> MNAHLANEVQYDLGHARVGPSSLVHVIISSECLAAAGIPLAALMRGRPGLGTAANFQVEIQTRAHATGDCTPWCTAFAAYVPADAVGELLAPVVPAHPGLLPRASSAGGLFVSLPVVCDAQGVYDPYAVAALRLAWGSGASCARVILFSYDELVPPNTRYAADSTRIMRVCRHLCRYVALLGAAAPPAAKEAAAHLSMGLGESASPRPQPLARPHAGAPADPPIVGASDPPISPEEQLTAPGGDTTAAQDVSIAQENEEILALVQRAVQDVTRRHPVRARTGRAACGVASGLRQGALVHQAVSGGAMGAADADAVLAGLEPPGGGRFVAPAPHGPGGEDILNDVLTLTPGTAKPRSLVEWLDRGWEALAGGDRPDWLWSRRSISVVLRHHYGTKQRFVVVSYENSVAWGGRRARPPLLSSALATALTEACAAERVVRPHQLSPAGQAELLLRFPALEVPLRHPRPVLPPFDIAAEVAFTARIHLACLRALGQAIRAALQGGPRISQRLRYDFGPDQRAWLGEVTRRFPILLENLMRAVEGTAPDAFFHTAYALAVLAHLGGRGGRGRRVVPLGDDLPARFADSDGHYVFDYYSTSGDTLRLNNRPIAVAMDGDVSKREQSKCRFMEAVPSTAPRRVCEQYLP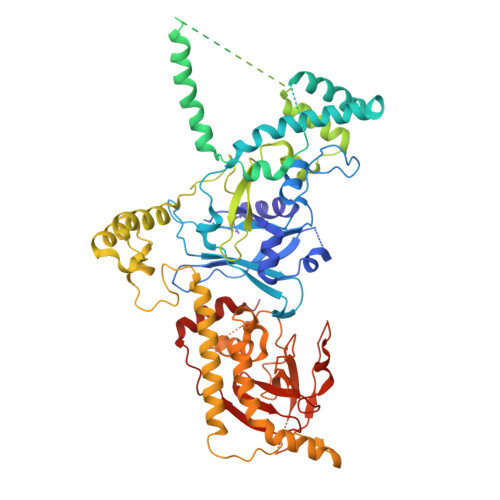GESYAYLCLGFNRRLCGIVVFPGGFAFTINIAAYLSLSDPVARAAVLRFCRKVS4-((R)-1-((R,Z)-6-(5-chloro-2-methoxybenzyl)-3-(ethoxyimino)-7-oxo-1,4-diazepane-1-carboxamido)propyl)benzoic 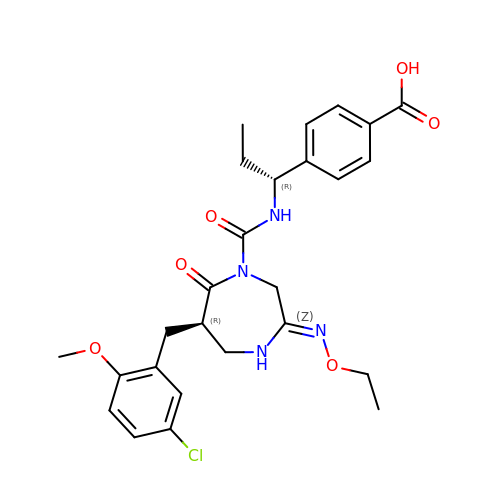acid | C26 H31 Cl N4 O6 | ZHZSQRPEOXQFJC-TZIWHRDSSA-N>MTATITDINAHEILDSRANPTLEVRVTLSSQAYGCAAVPSGASTGEREAVELRDNDLERYGGKGVLQAVENVNGPIRDALLGQDPRSQEEIDRIMIELDGTENKANLGANAILGVSLAVAYAAANNADLPLYRYLGGDGGPFSMPVPMMNIINGGAHATNNLDFQEFMIVPVGAPTFAEALRYGAEVFHALKKRLVSRGLMSAVGDEGGFAPDLPNNEAAFELILEAIEDANYVPGKDIYLALDAASSELYQNGRYDFENNQLTSEEMIDRLTEWTKKYPVISIEDGLSENDWAGWKLLTERLENKVQLVGDDIFVTNPDILEKGIKKNIANAILVKLNQIGTLTETLATVGLAKSNKYGVIISHRSGETEDTTIADLAVATDARQ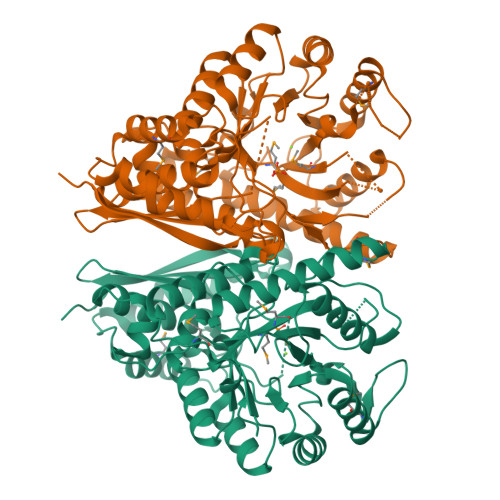IKTGSLCRSDRVAKYNRLLQIERELNDQAPYAGKEAFLFNRK[2x]>[2x]INDPAKSAAPYHDEFPLFRSANMASPDKLSTGIGFHSFRIPAVVRTTTGRILAFAEGRRHTNQDFGDINLVYKRTKTTANNGASPSDWEPLREVVGSGAGTWGNPTPVVDDDNTIYLFLSWNGATYS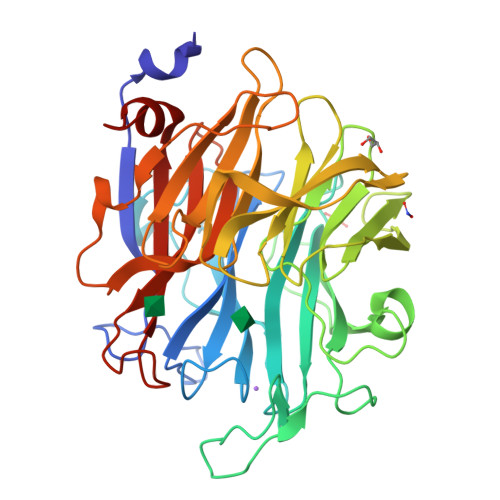QNGKDVLPDGTVTKKIDSTWEGRRHLYLTESRDDGNTWSKPVDLTKELTPDGWAWDAVGPGNGIRLTTGELVIPAMGRNIIGRGAPGNRTWSVQRLSGAGAEGTIVQTPDGKLYRNDRPSQKGYRMVARGTLEGFGAFAPDAGLPDPACQGSVLRYNSDAPARTIFLNSASGTSRRAMRVRISYDADAKKFNYGRKLEDAKVSGAGHEGGYSSMTKTGDYKIGALVESDFFNDGTGKNSYRAIIWRRFNLSWILNGPNN>[4x]MSRLLALLALAPLLAGAAETTAPKPPSAFTVEAQRRVEAELPFADRADFERADRGLIRRPERLLIRNPDGSVAWQLGGYDFLLDGKPRDSINPSLQRQALLNLKYGLFEVAEGIYQVRGFDLANITFIRGDSGWIVVDTLTTPATARAAYELVSRELGERPIRTVIYSHAHADHFGGVRGLVEPQQVASGAVQIIAPAGFMEAAIKENVLAGNAMMRRATYQYGTQLPKGPQGQVDMAIGKGLARGPLSLLAPTRLIEGEGEDLVLDGVPFTFQNTPGTESPAEMNIWLPRQKALLMAENVVGTLHNLYTLRGAEVRDALGWSKYINQALHRFGRQAEVMFAVHNWPRWGNAEIVEVLEKQRDLYG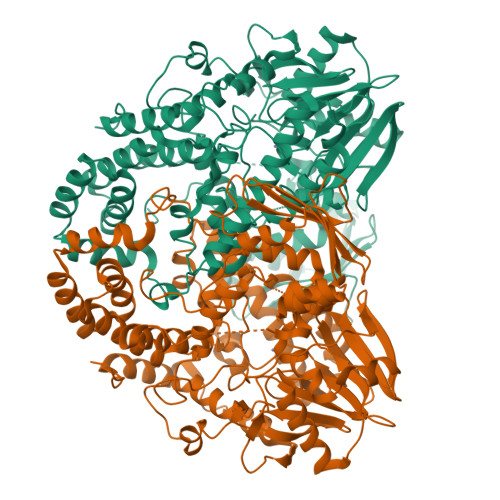YLHDQTLHLANQGVTIGQVHNRLRLPPSLDQEWYDRGYHGSVSHNARAVLNRYLGYYDGNPATLDPLSPEDSAGRYVEYMGGAERLLEQARASYARGEYRWVVEVVNRLVFAEPDNRAARELQADALEQLGYQAENAGWRNSYLSAAYELRHGVPRDQPTMKAGSADALAAMDTGLLFDYLGVRLDAGAAEGKALSINLRLPDIGENYLLELKNSHLNNLRGVQSEDAGQTVSIDRADLNRLLLKEVSAVRLVFEGKLKSSGNPLLLGQLFGMLGDFDFWFDIVTPAAKSEG> MKVAVLPGDGIGPEVTEAALKVLRALDEAEGLGLAYEVFPFGGAAIDAFGEPFPEPTRKGVEEAEAVLLGSVGGPKWGTGSVRPEQGLLSLRKSQDLFANLRPAKVFPGLERLSPLKEEIARGVDVLIVREL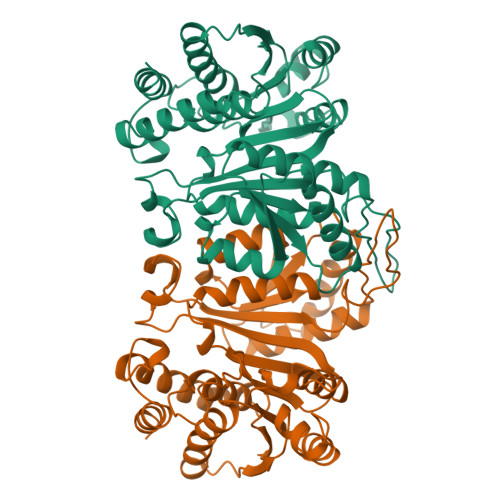TGGIYFGEPRGMSEAEAWNTERYSKPEVERVARVAFEAARKRRKHVVSVDKANVLEVGEFWRKTVEEVGRGYPDVALEHQYVDAMAMHLVRSPARFDVVVTGNIFGDILSDLASVLPGSLGLLPSASLGRGTPVFEPVHGSAPDIAGKGIANPTAAILSAAMMLEHAFGLVELARKVEDAVAKALLETPPPDLGGSAGTEAFTATVLRHLA> KGSVVIVGRIILS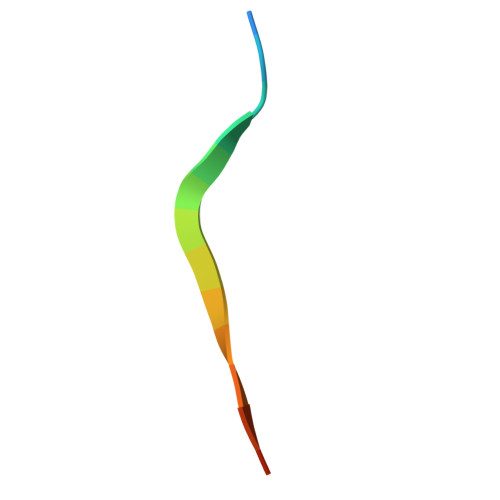GRK>MKTIEVDDELYSYIASHTKHIGESASDILRRMLKFSAASQPAAPVTKEVR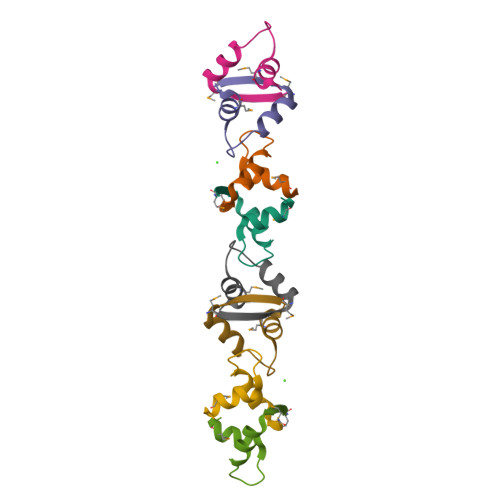[4x]>[3x]GAMGSMWKRSEQMKIKSGKCNMAAAMETEQLGVEIFETADCEENIESQDRPKLEPFYVERYSWSQLKKLLADTRKYHGYMMAKAPHDFMFVKRNDPDGPHSDRIYYLAMSGENRENTLFYSEIPKTINRAAVLMLSWKPLLDLFQATLDYGMYSREEELLRERKRIGTVGIASYDYHQGSGTFLFQAGSGIYHVKDGGPQGFTQQPLRPNLVETSCPNIRMDPKLCPADPDWIAFIHSNDIWISNIVTREERRLTYVHNELANMEEDARSAGVATFVLQEEFDRYSGYWWCPKAETTPSGGKILRILYEENDESEVEIIHVTS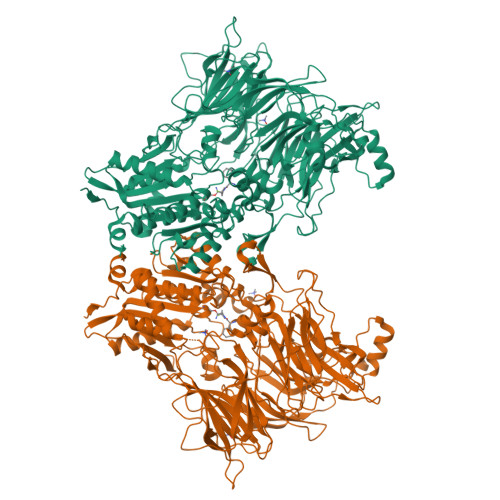PMLETRRADSFRYPKTGTANPKVTFKMSEIMIDAEGRIIDVIDKELIQPFEILFEGVEYIARAGWTPEGKYAWSILLDRSQTRLQIVLISPELFIPVEDDVMERQRLIESVPDSVTPLIIYEETTDIWINIHDIFHVFPQSHEEEIEFIFASECKTGFRHLYKITSILKESKYKRSSGGLPAPSDFKCPIKEEIAITSGEWEVLGRHGSNIQVDEVRRLVYFEGTKDSPLEHHLYVVSYVNPGEVTRLTDRGYSHSCCISQHCDFFISKYSNQKNPHCVSLYKLSSPEDDPTCKTKEFWATILDSAGPLPDYTPPEIFSFESTTGFTLYGMLYKPHDLQPGKKYPTVLFIYGGPQVQLVNNRFKGVKYFRLNTLASLGYVVVVIDNRGSCHRGLKFEGAFKYKMGQIEIDDQVEGLQYLASRYDFIDLDRVGIHGWSYGGYLSLMALMQRSDIFRVAIAGAPVTLWIFYDTGYTERYMGHPDQNEQGYYLGSVAMQAEKFPSEPNRLLLLHGFLDENVHFAHTSILLSFLVRAGKPYDLQIYPQERHSIRVPESGEHYELHLLHYLQENLGSRIAALKVI>SNRDLFAELSSALVEAKQHSEGKLTLKTHHVNDVGELNISPDEIVSIREQFNMSRGVFARLLHTSSRTLENWEQGRSVPNGQAVTL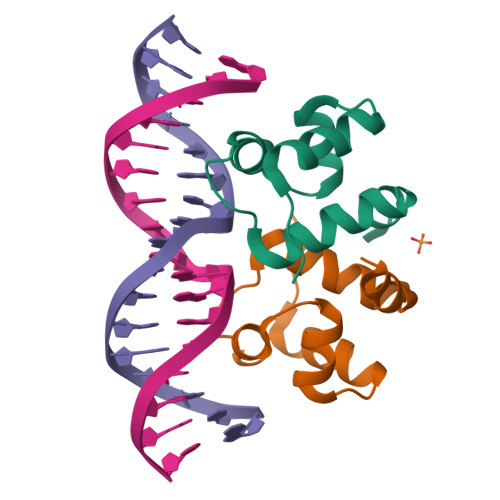LKLVQRHPETLSHIAEL[2x]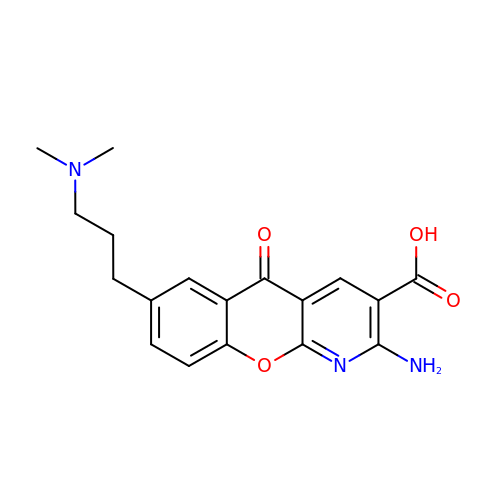2-amino-7-[3-(dimethylamino)propyl]-5-oxo-5H-[1]benzopyrano[2,3-b]pyridine-3-carboxylic acid | C18 H19 N3 O4 | UFHZMIKXSGTKFX-UHFFFAOYSA-N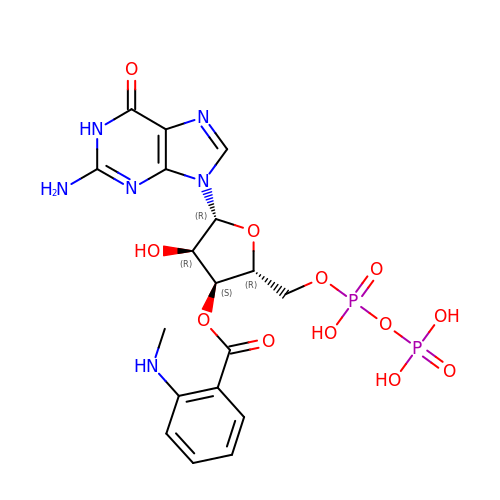3'-O-(N-methylanthraniloyl)guanosine-5'-diphosphate | C18 H22 N6 O12 P2 | DAJQUPOUYBWRQQ-XNIJJKJLSA-N> NYPAYMDNYLKEVINQVEEETGYNLLTTGMDVYTNVDQEAQKHLWDIYNTDEYVAYPDDELQVASTIVDVSNGKVIAQLGAR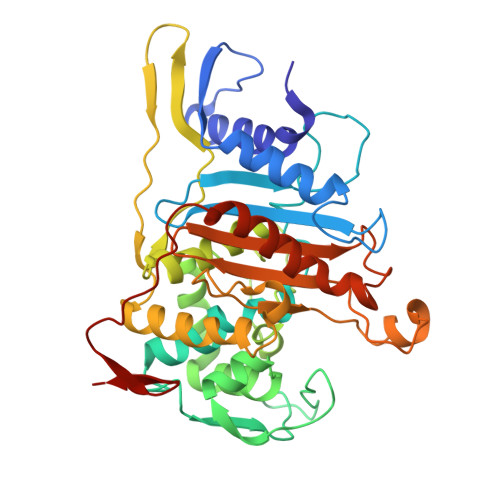HQSSNVSFGINQAVETNRDWGSTMKPITDYAPALEYGVYDSTATIVHDEPYNYPGTNTPVYNWDRGYFGNITLQYALQQSRNVPAVETLNKVGLNRAKTFLNGLGIDYPSIHYSNAISSNTTESDKKYGASSEKMAAAYAAFANGGTYYKPMYIHKVVFSDGSEKEFSNVGTRAMKETTAYMMTDMMKTVLTYGTGRNAYLAWLPQAGKTGTSNYTDEEIENHIKTSQFVAPDELFAGYTRKYSMAVWTGYSNRLTPLVGNGLTVAAKVYRSMMTYLSEGSNPEDWNIPEGLYRNGEFVFKN> MVPVEDLVYRYALLNAVKHRGRANPGAVMGAVMSNEPELRKMAPQVKEAVEAAVERVNSLSPEEQQQEMERLGLEITERKQKKRKGLRELAGVKGEVVLRFAPNPSGPLHIGHARAAILNHEYARKYDGRLILRIEDTDPRRVDPEAYDMIPADLEWLGVEWDETVIQSDRMETYYEYTEKLIERGGAYVCTCRPEEFRELKNRGEACHCRSLGFRENLQRWREMFEMKEGSAVVRVKTDLNHPNPAIRDWVSMRIVEAEHPRTGTRYRVYPMMNFSVAVDDHLLGVTHVLRGKDHLANREKQEYLYRHLGWEPPEFIHYGRLKMDDVALSTSGAREGILRGEYSGWDDPRLGTLRAIARRGIRPEAIRKLMVEIGVKIADSTMSWKKIYGLNRSILEEEARRYFFAADPVKL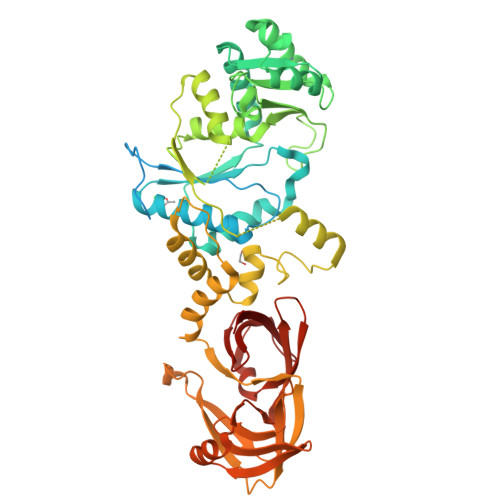EVVGLPGPVRVERPLHPDHPEIGNRVLELRGEVYLPGDDLGEGPLRLIDAVNVIYSGGELRYHSEGIEEARELGASMIHWVPAESALEAEVIMPDASRVRGVIEADASELEVDDVVQLERFGFARLDSAGPGMVFYYAHK>MQNERSEQSMPGMPAPGLPAGFERRFSRRYAQLDDVRLHYVTGGPDDGEMVVLLHGWPQTW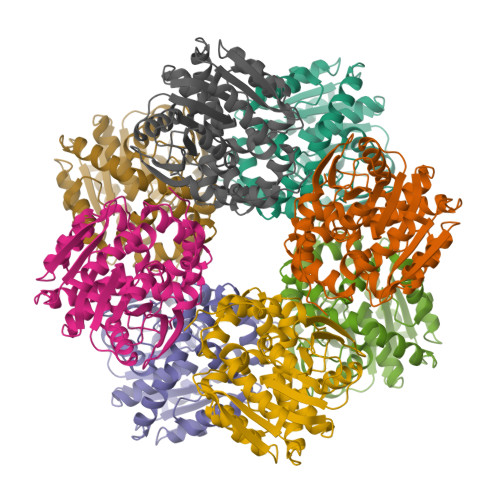YTWRHVMPALAEDGYRVVAVDYRGAGESDKPLGGYDKASMAGDIRALVHQLGATRIHLVGRDIGVMVAYAYAAQWPTEIVKLAMLDVPVPGTRIWDEAKASADPQIWHFGLHQQRDIAEMLIAGKERAYILDFYKKRTHVALSNDDIAVYADAYAAPGALRAGFELYRAFPQDETRFKAFMKHKLPMPVLALAGDKSNGAKELDMARELALDVRGAVAPNTGHWLPDENPAFLTRQLLDFFREAASGR[4x]> SIMTVRTTHTEVEVHAGGTVELPCSYQLANDTQPPVISWLKGASPDRSTKVFKGNYNWQGEGLGFVESDSYKESFGDFLGRASVANLAAPTLRLTHVHPQDGGRYWCQVAQWSIRTEFGLDAKSVVLKVTGHTPSNNVHVSTAEVVQVDEGNDITMTCPCTDCANANVTWYTGPTFFENYETGTYQPLANKNQFGITWFSSEI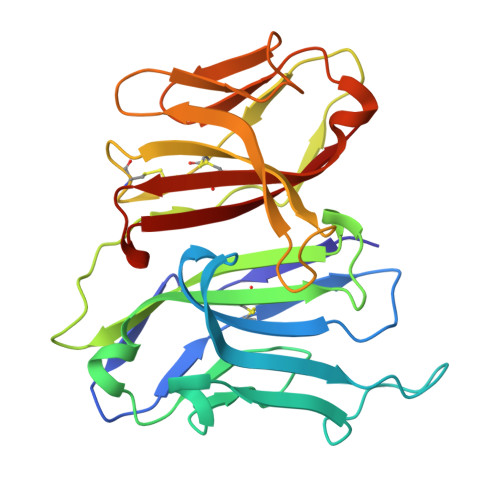AGRASFSGARNLVIRAAKITDAGRVWCELATGQGELDADRSSTILKV>[2x]MNKYTINDITRASGGFAMLAVDQREAMRMMFAAAGAPAPVADSVLTDFKVNAAKALSPYASAILVDQQFCYRQVVEQNAIAKSCAMIVAADEFIPGNGIPVDSVVIDRKINPLQIKQDG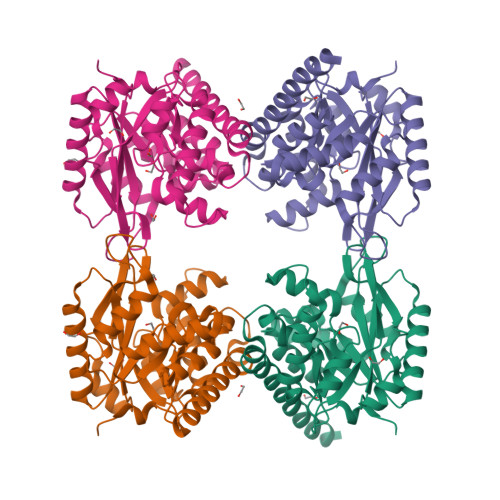GKALKLLVLWRSDEDAQQRLDMVKEFNELCHSHGLVSIIEPVVRPPRRGDKFDREQAIIDAAKELGDSGADLYKVEMPLYGKGPQQELLCASQRLNDHINMPWVILSSGVDEKLFPRAVRVAMTAGASGFLAGRAVWASVVGLPDNELMLRDVCAPKLQQLGDIVDEMMAKRRLEHHHHHH~{N}-[3-[[4-[bis(fluoranyl)methoxy]phenyl]sulfamoyl]phenyl]-3,5-bis(fluoranyl)benzamide | C20 H14 F4 N2 O4 S | 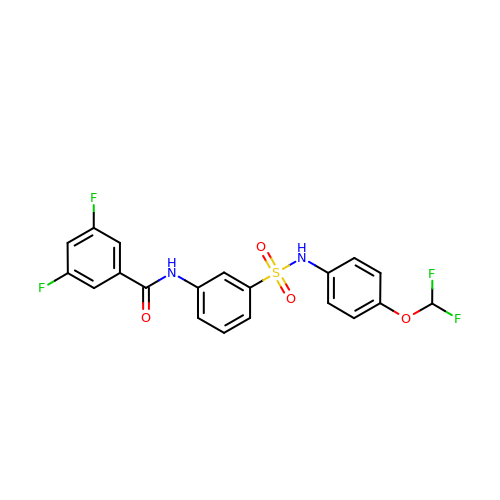RCXBNPJQQXMWGZ-UHFFFAOYSA-N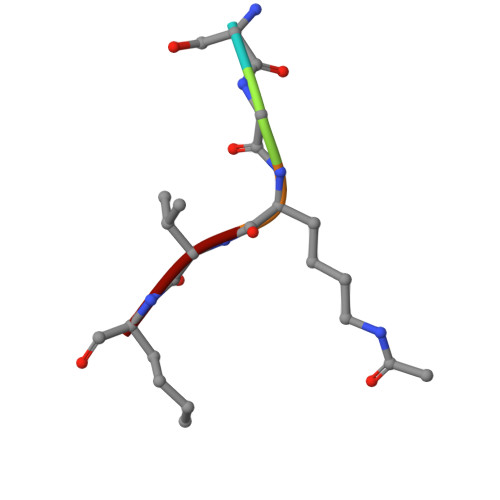> SGKVL1-tert-butyl-3-naphthalen-2-yl-1H-pyrazolo[3,4-d]pyrimidin-4-amine 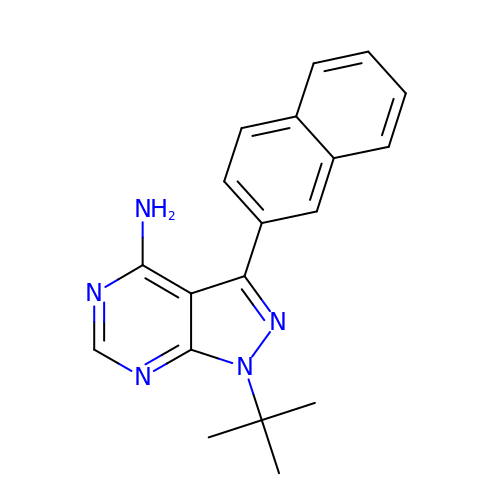| C19 H19 N5 | ILKDWZKZLIHMFM-UHFFFAOYSA-N>SVKISDDISITQLSDKVYTYVSLAEIEGWGMVPSNGMIVINNHQAALLDTPINDAQTEMLVNWVTDSLHAKVTTFIPNHWHGDCIGGLGYLQRKGVQSYANQMTIDLAKEKGLPVPEHGFTDSLTVSLDGM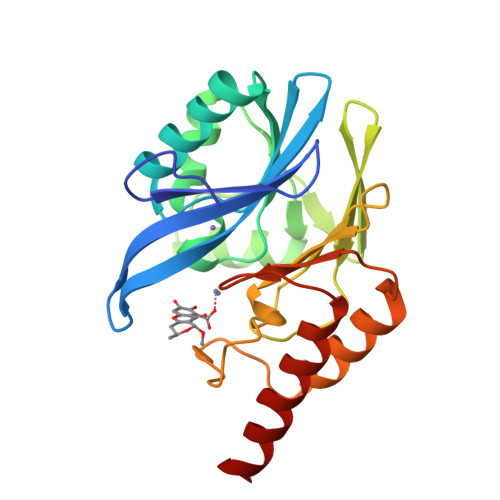PLQCYYLGGGHATDNIVVWLPTENILFGGCMLKDNQATSIGNISDADVTAWPKTLDKVKAKFPSARYVVPGHGDYGGTELIEHTKQIVNQYIESTS[2x]NEOMYCIN 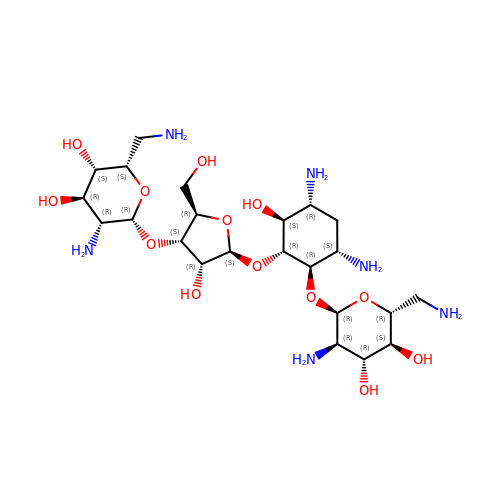| C23 H46 N6 O13 | PGBHMTALBVVCIT-VCIWKGPPSA-N> MAKPCGVRLSGEARKQVDVFRQNLFQEADDFLCTFLPRKIISLS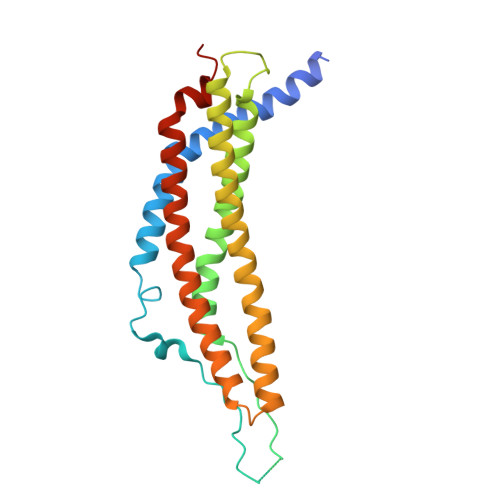QLLQEDSLNVADLSSLRAPLDIPIPDPPPKDDEMETDKQEKKEVPKCGYLPGNEKLLALLALVKPEVWTLKEKCILVITWIQHLIPKIEDGNDFGVAIQEKVLERVNAVKTKVEAFQTTISKYFSERGDAVAKASKDTHVMDYRALVHERDEAAYGALRAMVLDLRAFYAELYHIISSNLEKIVNPKGEEKPSMY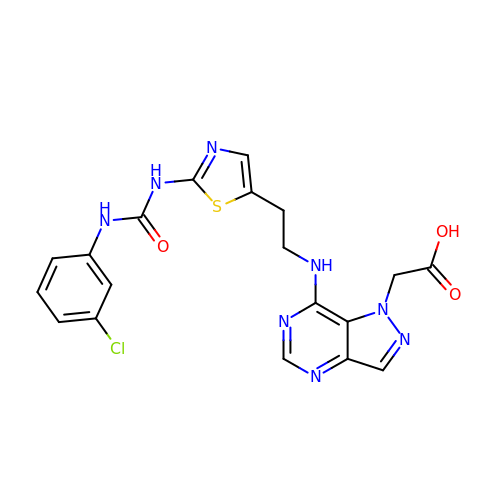(7-{[2-(2-{[(3-chlorophenyl)carbamoyl]amino}-1,3-thiazol-5-yl)ethyl]amino}-1H-pyrazolo[4,3-d]pyrimidin-1-yl)acetic acid | C19 H17 Cl N8 O3 S | WRGKHKVUWQKICT-UHFFFAOYSA-N> GSKEGEYIKLKVIGQDSSEIHFKVKMTTHLKKLKESYAQRQGVPM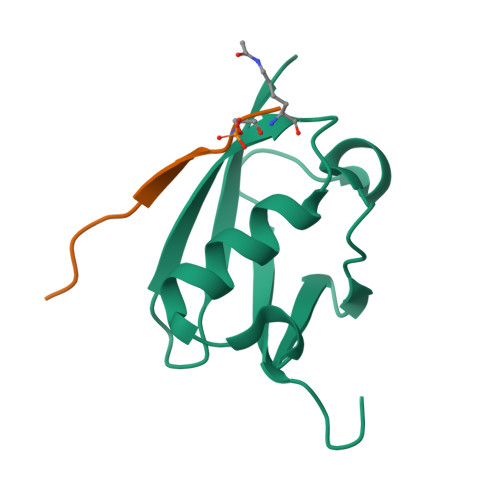NSLRFLFEGQRIADNHTPKELGMEEEDVIEVYQEQTGG;> GSGEAEERIIVLSDSDY>NSRTVLILCGDYMEDYEVMVPFQALQAFGITVHTVCPGKKAGDSCPTAVHDFCGHQTYFESRGHNFTLNATFDEVDLSKYDGLVIPGGRAPEYLALTASVVELVKEFSRSGKPIASIXHGQLILAAADTVNGRKCTAYATVGPSLVAAGAKWVEPITPDVCVVDGSLITAATYEGHPEFIQLFVKALGGKITGANKRILFLCGDYMEDYEVKVPFQSLQALGCQVDAVCPEKKAGDRCPTAIHDFEGDQTYSEKPGHTFALTTNFDDLVSSSYDALVIPGGRAPEYLALNEHVLNIVKEFMNSEK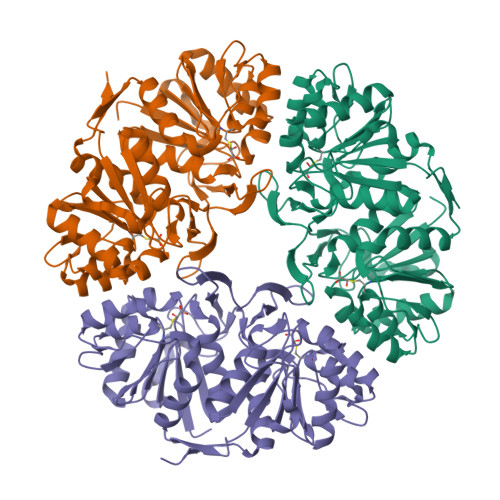PVASIXHGQQILAAAGVLKGRKCTAYPAVKLNVVLGGGTWLEPDPIDRCFTDGNLVTGAAWPGHPEFVSQLMALLGIQVSFHH[3x]>PAMTSSDLPLNFQGSPCSQIWQHPRFAAKKRSSMVKFHCYTNHSGALTWFRKRGSQQPQELVSEEGRIVQTQNGSVYTLTIQNIQYEDNGIYFCKQKCDSANHNVTDSCGTELLVLGFSTLDQL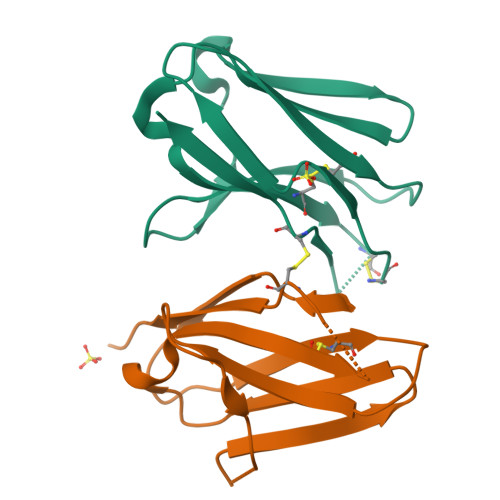KRRNTLKDG[2x]> MAHHHHHHMVPDSRKAAVLGSPITHSRSPQLHLAAYRALGLPSWTYERIECTAEQLPGLVSALGPEWVGLSVTMPGKFAALEFADQRTDRAQLVGSANTLVRMPTGGWRADNTDVDGVTGALGTAGDSALVIGSGGTAPAAVVALAELGVQRITIVARDEGKASRLVDLARRCGAQGGWCDIGGAALADAVASADAAVSTIPADAAA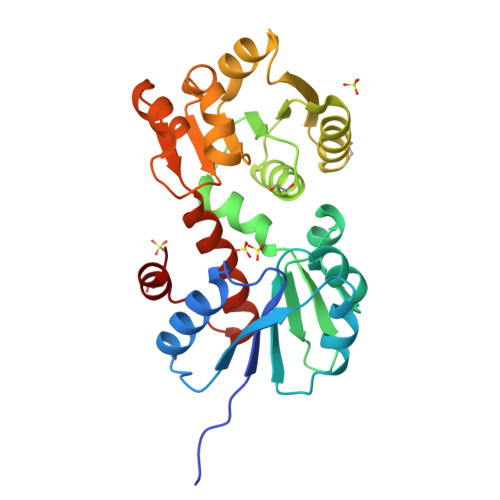VYADALARVPRVLDAIYDPWPTPLAQAVEAAGGEAINGLQMLLNQAFAQVEQFTGMPAPKEAMRAALG>[2x]MTSLFTTADHYHTPLGPDGTPHAFFE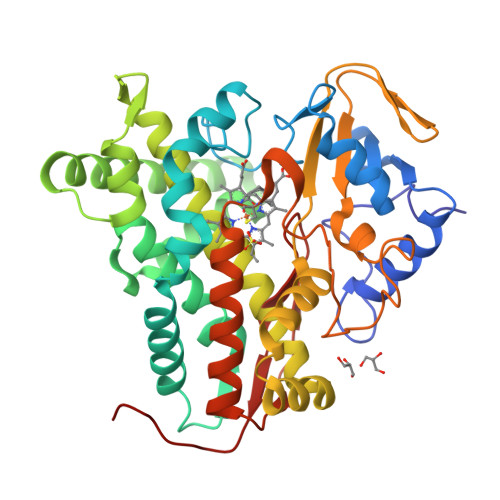ALRDEAETTPIGWSEAYGGHWVVAGYKEIQAVIQNTKAFSNKGVTFPRYETGEFELMMAGQDDPVHKKYRQLVAKPFSPEATDLFTEQLRQSTNDLIDARIELGEGDAATWLANEIPARLTAILLGLPPEDGDTYRRWVWAITHVENPEEGAEIFAELVAHARTLIAERRTNPGNDIMSRVIMSKIDGESLSEDDLIGFFTILLLGGIDNTARFLSSVFWRLAWDIELRRRLIAHPELIPNAVDELLRFYGPAMVGRLVTQEVTVGDITMKPGQTAMLWFPIASRDRSAFDSPDNIVIERTPNRHLSLGHGIHRCLGAHLIRVEARVAITEFLKRIPEFSLDPNKECEWLMGQVAGMLHVPIIFPKGKRLSE N-BENZYLFORMAMIDE | C8 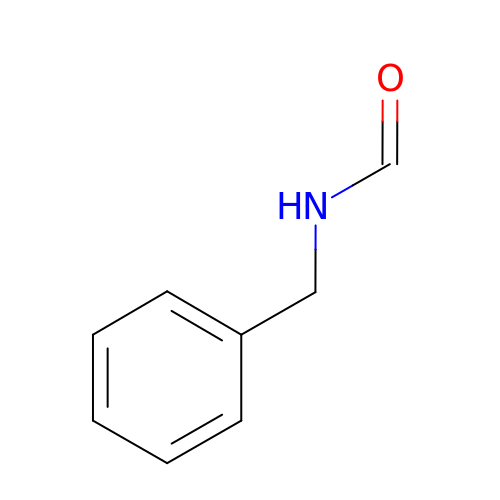H9 N O | IIBOGKHTXBPGEI-UHFFFAOYSA-N> MGSPASDPTVFHKRYLKKIRDLGEGHFGKVSLYCYDPTNDGTGEMVAVK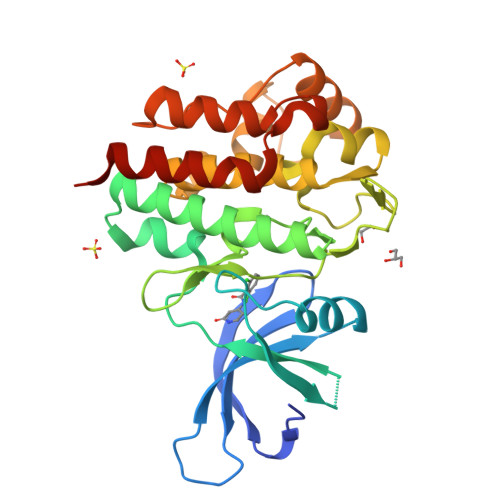ALKADCGPQHRSGWKQEIDILRTLYHEHIIKYKGCCEDQGEKSLQLVMEYVPLGSLRDYLPRHSIGLAQLLLFAQQICEGMAYLHSQHYIHRNLAARNVLLDNDRLVKIGDFGLAKAVPEGHEYYRVREDGDSPVFWYAPECLKEYKFYYASDVWSFGVTLYELLTHCDSSQSPPTKFLELIGIAQGQMTVLRLTELLERGERLPRPDKCPCEVYHLMKNCWETEASFRPTFENLIPILKTVHEKYRHHHHHH>MANTGSLVLLRHGESDWNALNLFTGWVDVGLTDKGQAEAVRSGELIAEHDLLPDVLYTSLLRRAITTAHLALDSADRLWIPVRRSWRLNERHYGALQGLDKAETKARYGEEQFMAWRRSYDTPPPPIERGSQFSQDADPRYADIGGGPLTECLADVVARFLPYFTDVIVGDLRVGKTVLIVAHGNSLRALVKHLDQMSDDEIVGLNIPTGIP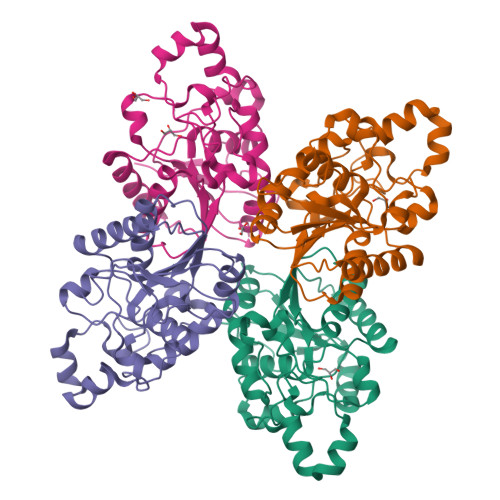LRYDLDSAMRPLVRGGTYLDPEAAAAGAAAVAGQGRGGVPRGAAALEHHHHHH[4x]> DDKMDYDFKVKLSSERERVEDLFEYEGCKVGRGTYGHVYKAKRKDGKDDKDYALKQIEGTGISMSACREIALLRELKHPNVISLQKVFLSHADRKVWLLFDYAEHDLWHIIKFHRASKANKKPVQLPRGMVKSLLYQILDGIHYLHANWVLHRDLKPANILVMGEGPERGRVKIADMGFARLFNSPLKPLADLDPVVVTFWYRAPELLLGARHYTKAIDIWAIGCIFAELLTSEPIFHCRQEDIKTSNPYHHDQLDRIFNVMGFPADKDWEDIKKMPEHSTLMKDFRRNTYTNCSLIKYMEKHKVKPDSKAFHLLQKLLTMDPIKRITSEQAMQDPYFLEDPLPTSDVFAGCQIPYPKREFLTEEEPDDKGDKKNQQQQQGNNHTNGTGHPGNQDSSHTQGPPLKK;> KAMAGNFWQSSHYLQWILDKQDLLKERQKDLKFLSEEEYWKLQIFFTNVIQALGEHLKLRQQVIATATVYFKRFYARYSLKSIDPVLMAPTCVFLASKVEEFGVVSNTRLIAAATSVLKTRFSYAFPKEFPYRMNHILECEFYLLELMDCCLIVYHPYRPLLQYVQDMGQEDMLLPLAWRIVNDTYRTDLCLLYPPFMIALACLHVACVVQQKDARQWFAELSVDMEKILEIIRVILKLYEQWKNFDERKEMATILSKMPKPKPP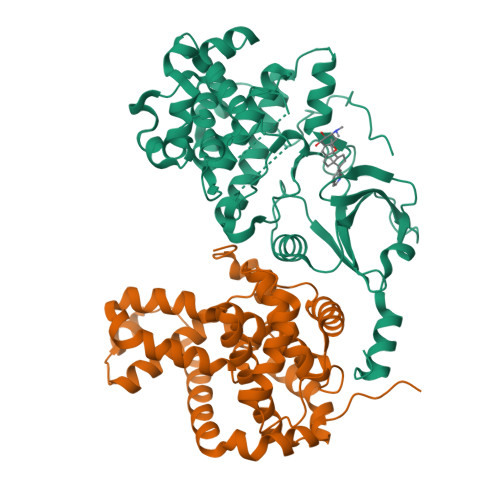PNSEGEQGPNGSQNSSYSQS> ACLSRIDANLLQYYEKPEPNNTVDLYVSNNSNNNGLKEGDKSISTPVPQPYGSEYSNCLLLSNSEYICYHFSSRSTLLTFYPLSDAYHGKTINIHLPNASMNQRYTLTIQEVEQQLLVNVILKDGSFLTLQLPLSFLFSSANTLNGEWFHLQNPYDFTVRVPHFLFYVSPQFSVVFLEDGGLLGLKKVDGVHYEPLLFNDNSYLKSLTRFFSRSSKSDYDSVISCKLFHERYLIVLTQNCHLKIWDLTSFTLIQDYDMVSQSDSDPSHFRKVEAVGEYLSLYNNTLVTLLPLENGLFQMGTLLVDSSGILTYTFQNNIPTNLSASAIWSIVDLVLTRPLELNVEASYLNLIVLWKSGTASKLQILNVNDESFKNYEWIESVNKSLVDLQSEHDLD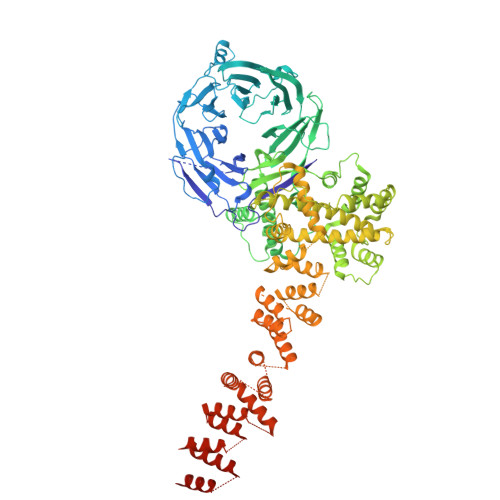IVTKTGDVERGFCNLKSRYGTQIFERAQQILSENKIIMAHNEDEEYLANLETILRDVKTAFNEASSITLYGDEIILVNCFQPYNHSLYKLNTTVENWFYNMHSETDGSELFKYLRTLNGFASTLSNDVLRSISKKFLDIITGELPDSMTTVEKFTDIFKNCLENQFEITNLKILFDELNSFDIPVVLNDLINNQMKPGIFWKKDFISAIKFDGFTSIISLESLHQLLSIHYRITLQVLLTFVLFDLDTEIFGQHISTLLDLHYKQFLLLNLYRQDKCLLAEVLLKDSSEFSFGVKFFNYGQLIAYIDSLNSNVYNASITENSFFMTFFRSYIIENTSHKNIRFFLENVECPFYLRHNEVQEFMFAMTLFSCGNFDQSYEIFQLHDYPEAINDKLPTFLEDLKSENYHGDSIWKDLLCTFTVPYRHSAFYYQLSLLFDRNNSQEFALKCISKSAEYSLKEIQIEELQDFKEKQHIHYLNLLIHFRMFEEVLDVLRLGHECLSDTVRTNFLQLLLQEDIYSRDFFSTLLRLCNAHSDNGELYLRTVDIKIVDSILSQNLRSGDWECFKKLYCFRMLNKSERAAAEVLYQYILMQADLDVIRKRKCYLMVINVLSSFDSAYDQWILNGSKVVTLTDLRDELRG>MKIGANYTPSQGWFHSWLDLDIDATRRDFEGIAQLGLDHVRLFPLWPLLQPNRGLVRPRALDDVVSVVRAAGEFDLE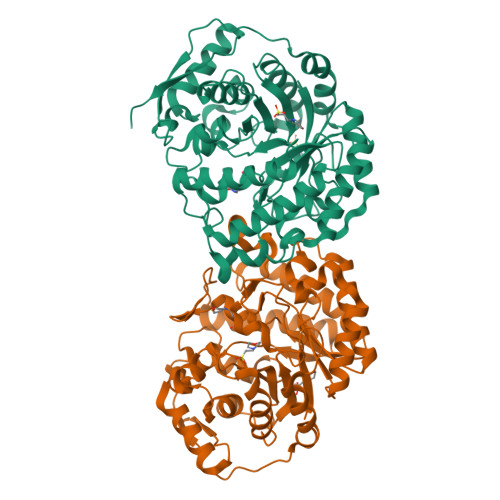VTVDALNGHLSSYDFLPPWVITWHTSNLFTDPLVKAGQTDLISQLATRLREEPNATGMTVGNEFPQYAALAPGHHHPTRSECTVDDAQTWLETMLGTMRDQWPDGRFWFGFDDDLWFVDDHPFTPRHAVTQGSATTVHSWVFAQVGPRFGEGHPALTWFPRYLLELARAWSHDPERPLWLQEVGAPRTHVPDSSSAAFMTTTMASLTSTPGLEAITWWCSHDVSRDLLDFPELEYSLGLFTNDGKPKPEALALSDMLPDLHNAQPQHQLDEPLEFSANWDTGAGRSVCSPMGDLFAQWVDQAEQTGRAPRLALRPTPGLTDREALASARAHSAHHHHHH[4x]>[2x]GGNQVQIKVLNIGNNNMTVHFPGNSVTLAQMSQTDTFMTFDIDKLTSINI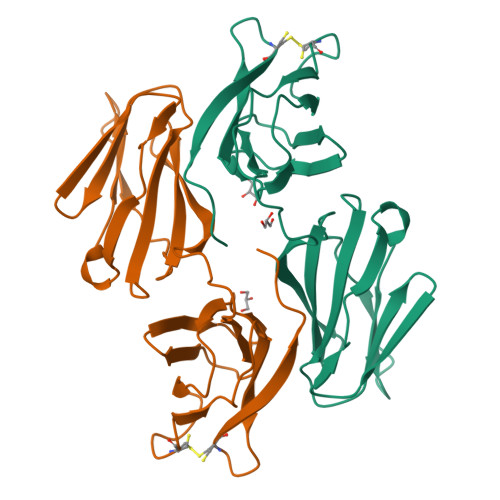SSSGSPGVTTVAHDFEQGHRHTLLVWNPSQYRVVKDGLNQKPEKGENGIRFVNTLNEMVTIKMSGKVYENVTSHNASGYQFFPSGEKQYTINTTAVAPTCLTDFKSSNLDFGSAYTYVIRRASDGCLEVKEFEDIPPNT>MSQLALQMSSLGVEGEGIWLALGTIGMLLGMLYFIADGLDVQDPRQKEFYVITILIPAIAAASYLSMFFGFGLTEVSLANGRVVDVYWARYADWLFTTPLLLLDIGLLAGASQRDIGALVGIDAFMIVTGLVATLTKVVVARYAFWTISTISMVFLLYYLVAVFGEAVSDADEDTRSTFNALRNIILVTWAIYPVA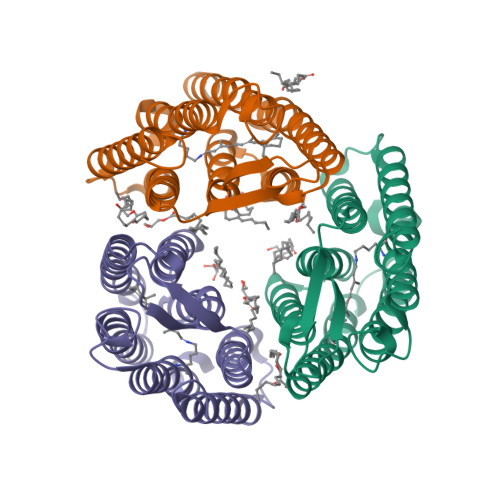WLVGTEGLALTGLYGETLLFMVLDLVAKVGFGFILLRSRAIMGGGSEPTPSAQETAADLVPRGSLEHHHHHH[3x]> GGGGUGUGCCCGGCAUGGGUGCAGUCUAUAGGGUGAGAGUCCCGAACUGUGAAGGCAGAAGUAACAGUUAGCCUAACGCAAGGGUGUCCGUGGCGACAUGGAAUCUGAAGGAAGCGGACGGCAAACCUUCGGUCUGAGGAACACGAACUUCAUAUGAGGCUAGGUAUCAAUGGAUGAGUUUGCAUAACAAAACAAAGUCCUUUCUGCCAAAGUUGGUACAGAGUAAAUGAAGCAGAUUGAUGAAGGGAAAGACUGCAUUCUUACCCGGGGAGGUCUGGAAACAGAAGUCAGCAGAAGUCAUAGUACCCUGUUCGCAGGGGAAGGACGGAACAAGUAUGGCGUUCGCGCCUAAGCUUGAACCGCCGUAUACCGAACGGUACGUACGGUGGUGUGG

The self-splicing group II introns are bacterial and organellar ancestors of the nuclear spliceosome and retro-transposable elements of pharmacological and biotechnological importance. Besides catalyzing their self-splicing, group II introns also act as mobile retroelements, thus crucially contributing to genetic diversity throughout evolution. Integrating enzymatic, crystallographic, and simulation studies, we demonstrate how these introns recognize small molecules through their conserved active site. These RNA-binding small molecules selectively inhibit the two steps of splicing by adopting distinctive poses at different stages of catalysis, and by preventing crucial active site conformational changes that are essential for splicing progression.

In the intronistat B-bound state the intron active site is intact and adopts the catalytically required triple helix conformation anchored to the M1/M2/K1 metal ion cluster. While the electron density around the metal cluster in the active site is weak, the interatomic distances and coordination spheres were compatible with magnesium ions at the M1 and M2 positions and with potassium ions at the K1 position. To localize the compound in the crystallographic electron density, we calculated the Fo-Fc electron density omit-map of the refined structure before modeling the ligand. The map shows an extended positive peak in the active site (highest contour value = 4.5 σ, volume of the peak at 3.0 σ = 449 Å3), compatible with the chemical structure and molecular volume of intronistat B (predicted volume of intronistat B = 333 Å3). Here, intronistat B makes specific contacts through its pyrogallol group with both M1 (2.0 Å from intronistat B O24 and O26 atoms) and M2 (2.0 Å from intronistat B O22 and O24 atoms). As shown by our quantum-level calculations, this binding mode is possible, because intronistat B is deprotonated at the hydroxyl group in para in the pyrogallol moiety (pKA = 5.7), analogously to other similar chelating groups. The pyrogallol moiety makes further hydrogen bond interactions with evolutionarily-conserved active site nucleotides, i.e. the catalytic triad and the 2-nucleotide bulge. Additionally, intronistat B establishes a sequence-specific hydrogen bond with exon binding site 1 (EBS1), the motif that recognizes the exon sequence and thus defines the splicing site (3.0 Å between O18 in intronistat B and N1 in A181). Finally, intronistat B also binds the exon-free intron by establishing contacts with the catalytic metal ions and both sequence-specific and sequence-unspecific interactions (conformation B).>[4x]GAMGNHKAALTKQVFTFASELYAYGVREVVISPGSRSTPLALAFEAHPNIKTWIHPDERSAAFFAVGLIKGSERPVAILCTSGTAAANYTPAIAESQISRIPLIVLTSDRPHELRSVGAPQAINQVNMFNNYVSYEFDMPIADDSKETINAIYYQMQIASQYLYGPHKGPIHFNLPFRDPLTPDLNATELLTSEMKILPHYQKSIDASALRHILNKKKGLIIVGDMQHQEVDQILTYSTIYDLPILADPLSHLRKFDHPNVICTYDLLFRSGLDLNVDFVIRVGKPVISKKLNQWLKKTD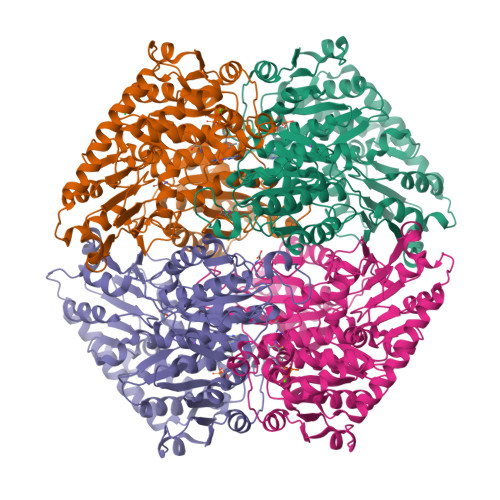AFQILVQNNDKIDVFPIAPDISYEISANDFFRSLMEDTTINRVSWLEKWQCLEKKGRKEIKCYLEQATDESAFVGELIKKTSEKDALFISNSMPIRDVDNLLLNKNIDVYANRGANGIDGIVSTALGMAVHKRITLLIGDLSFYHDMNGLLMSKLNNIQMNIVLLNNDGGGIFSYLPQKESATDYFERLFGTPTGLDFEYTAKLYQFDFKRFNSVSEFKNATLLSETSTIYELITNREDNFKQHQILYQKLSEMIHDTL> HHNGTNGTMMQYFEWYLPNDGNHWNRLNSDASNLKSKGITAVWIPPAWKGASQNDVGYGAYDLYDLGEFNQKGTVRTKYGTRSQLQAAVTSLKNNGIQVYGDVVMNHKGGADATEMVRAVEVNPNNRNQEVTGEYTIEAWTRFDFPGRGNTHSSFKWRWYHFDGVDWDQSRRLNNRIYKFRGHGKAWDWEVDTENGNYDYLMYADIDMDHPEVVNELRNWGVWYTNTLGLDGFRIDAVKHIKYSFTRDWINHVRSATGKNMFAVAEFWKNDLGAIENYLQKTNWNHSVFDVPLH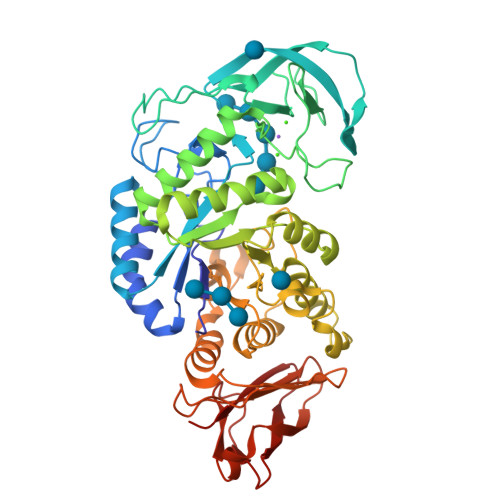YNLYNASKSGGNYDMRNIFNGTVVQRHPSHAVTFVDNHDSQPEEALESFVEEWFKPLAYALTLTREQGYPSVFYGDYYGIPTHGVPAMRSKIDPILEARQKYAYGKQNDYLDHHNIIGWTREGNTAHPNSGLATIMSDGAGGSKWMFVGRNKAGQVWSDITGNRTGTVTINADGWGNFSVNGGSVSIWVNK> MAHHHHHHMTQGLLAGKRFLIAGVASKLSIAYGIAQALHREGAELAFTYPNEKLKKRVDEFAEQFGSKLVFPCDVAVDAEIDNAFAELAKHWDGVDGVVHSIGFAPAHTLDGDFTDVTDRDGFKIAHDISAYSFVAMARAAKPLLQARQGCLLTLTYQGSERVMPNYNVMGMAKASLEAGVRYLASSLGV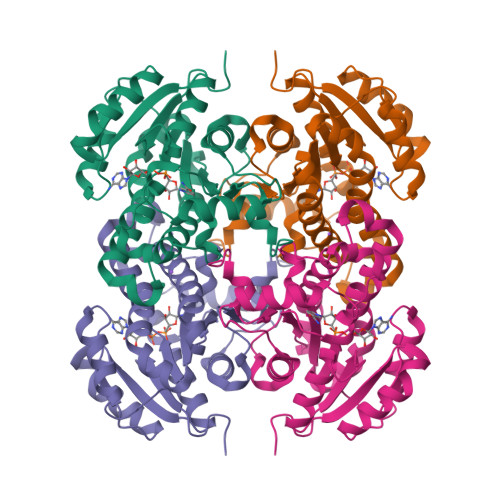DGIRVNAISAGPIRTLAASGIKSFRKMLDANEKVAPLKRNVTIEEVGNAALFLCSPWASGITGEILYVDAGFNTVGMSQSMMDDE Thiamine Triphosphate | C12 H20 N4 O10 P3 S | 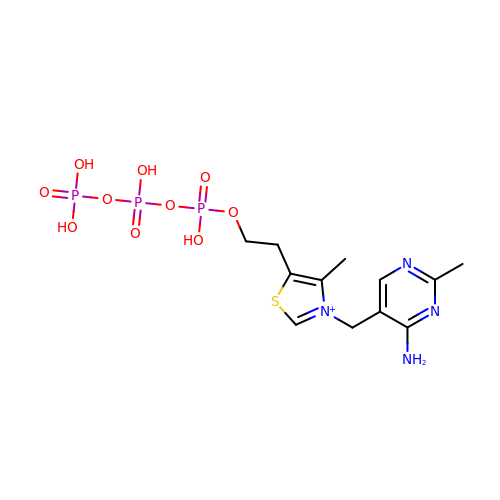IWLROWZYZPNOFC-UHFFFAOYSA-O1,5-ANHYDRO-2-C-(CARBOXYMETHYL-N-HYDROXYAMIDE)-2-DEOXY-3-O-MYRISTOYL-D-GLUCITOL 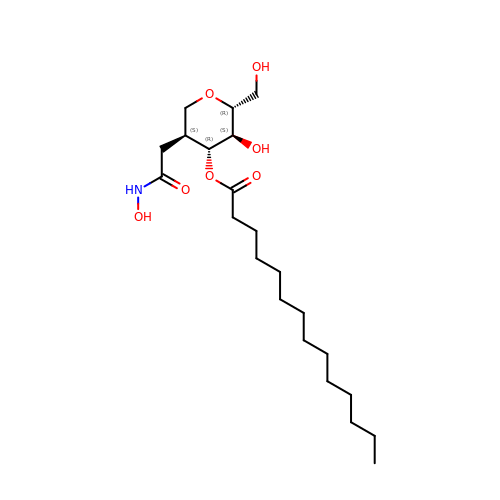| C22 H41 N O7 | INAPDIIIYSWKOC-XHIHJMKYSA-N> MADNMTTTQIEVGPGATNATINFEAGILECYERFSWQRALDYPGQD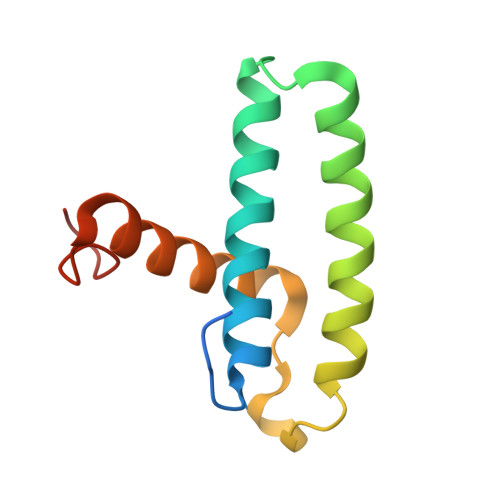RLHRLKRKLESRIKTHNKSEPENKRMSLEERKAIGVKMMKVLLFMDPSAGIEGFEPY>MLTPPPDSKISTTDKSLDKLSAPLDMLKQMNESTMEQTKLDELRKKMSLQAEILNKAKADNDMFFRLLIELMSLKLQGELFKEQLSKISKESGYDSAQSALIQATNSEGQSPLQYALQKQDFSTAKYFLDNGAKAGPIEKAVFEIALDSKAAKEFGFPPLPPEKEKLHPVKNFGLVLGIKTTSVDGTPSQFGHIAPTYQLMTDSVSHFAKSHPGNKNFQEIANAFQFSNEASAFKFSTPQRNPEAGNDLARRIQGGELTTIPVSCKGHAMGLSYVPDGPGSKSGYLVYTNRGLGAKSSEHGTHIFRIEDSSKITPEFINNMTSGHSNGASHDEIMSQIKAAAGNKEPIHHIKQKGQKNDNCTIANSKSNIEGILLCQKAREVGGFDKLTESDMDSVKKEYKEFTKHMRVEKVNELAKALKENPQDPDLNNLTKEYLKQHPNADPKLKQTLETALKQASESSMTLSQPGKTI[2x]

A Legionella effector LegA15, also known as AnkD, is one of 11 ankyrin repeat–containing effectors in L. pneumophila. The Dot/Icm effector LegA15, a 471–amino acid protein encoded by gene lpg2456 of L. pneumophila Philadelphia, harbors an ankyrin repeat (ANK) domain that is known to mediate protein-protein interactions in eukaryotic cells. LegA15 is a GTPase with a unique catalytic mechanism, unlike any eukaryotic small GTPases. Here, we show that an ankyrin repeat containing effector LegA15 localizes directly in host lipid droplets (LDs), leading to Golgi apparatus fragmentation of the host cells by hijacking the host vesicular transport factor p115.

We next solved a binary structure of LegA15 bound with an unhydrolyzable GTP analog 5′-guanylyl imidodiphosphate (GDPNP) at a resolution of 2.27 Å. GDPNP was well defined by its electron density. GDPNP is shown to bind a positive-charged pocket formed by Arg291, Arg408, and Lys367 without inducing a large conformational change of LegA15 because LegA15 in this complex is well aligned to its ligand-free form [root mean square deviation (RMSD) of 1.0 Å]. GDPNP also makes additional interactions with LegA15. The guanosine hydrogen bonds with residues of Gln353, Lys354, Ser368, and Tyr400 in addition to Lys367. The γ-phosphate of GTP is anchored by Ala364 and Gln356 via hydrogen bonds, while its β-phosphate hydrogen bonds with both Arg291, Gln356, and Lys367. The α-phosphate hydrogen bonds with Lys367. In addition, highly conserved residues Cys361 and Thr362 possibly interact with the γ-phosphate of GDPNP through an intermediate water, which is in a good position for a nucleophilic attack. Consistently, we observed that the C361S mutation retained the GTP binding but abolished the GTPase activity.>DPAVTYYRLEEVAKRNTAEETWMVIHGRVYDITRFLSEHPGGEEILLEQAGADATESFEDIGHSPD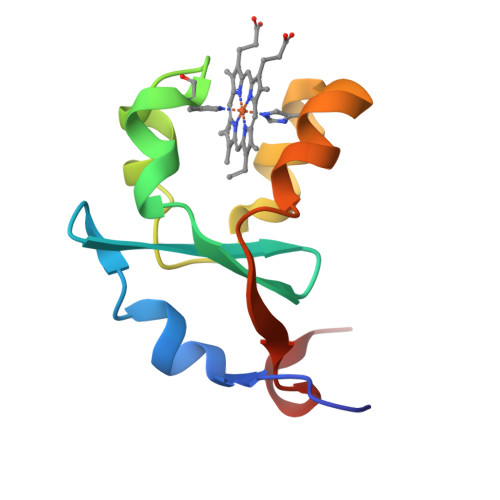AREMLKQYYIGDVHPNDLKP[2x]>MVPISPIETVPVKLKPGMDGPKVKQWPLTEEKIKALVEICTEMEKEGKISKIGPENPYNTPVFAIKKKDSTKWRKLVDFRELNKRTQDFWEVQLGIPHPAGLKQKKSVTVLDVGDAFYSVPLDKDFRKYTAFTIPSINNETPGIRYQYNVLPMGWKGSPAIFQSSMTKILEPFRKQNPDIVIYQYVDDLYVGSDLEIGQHRTKIEELRQHLLRWGFTTPDKKHQKEPPFLWMGYELHPDKWTVQPIVLPEKDSWTVNDIQKLVGKLNWASQIYAGIKVRQLSKLLRGTKALTEVVPLTEEAELELAENREILKEPVHGVYYDPSKDLIAEIQKQGQGQWTYQIYQEPFKNLKTGKYARMKGAHTNDVKQLTEAVQKIATESIVIWGKTPKFKLPIQKETWEAWWTEYWQATWIPEWEFVNTPPLVKLWYQLEKEPIIGAETFYVDGAANRETKLGKAGYVTDRGRQKVVPLTDTTNQKTELQAIHLALQDSGLEVNIVTDSQYALGIIQAQPDKSESELVSQIIEQLIKKEKVYLAWVPAHKGIGGNEQVDKLVSAG[2x];>[2x]MAHHHHHHALEVLFQGPISPIETVPVK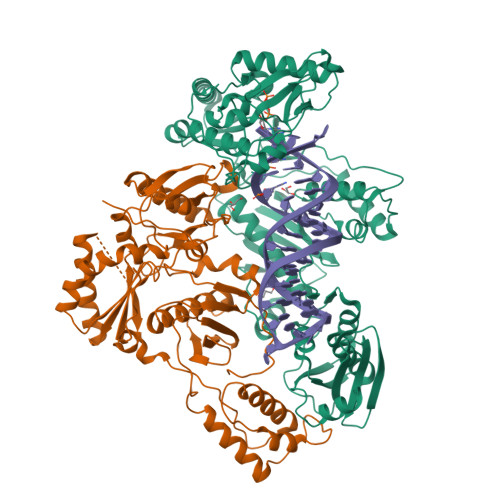LKPGMDGPKVKQWPLTEEKIKALVEICTEMEKEGKISKIGPENPYNTPVFAIKKKDSTKWRKLVDFRELNKRTQDFWEVQLGIPHPAGLKQKKSVTVLDVGDAYFSVPLDKDFRKYTAFTIPSINNETPGIRYQYNVLPQGWKGSPAIFQSSMTKILEPFRKQNPDIVIYQYMDDLYVGSDLEIGQHRTKIEELRQHLLRWGFTTPDKKHQKEPPFLWMGYELHPDKWTVQPIVLPEKDSWTVNDIQKLVGKLNWASQIYAGIKVRQLSKLLRGTKALTEVVPLTEEAELELAENREILKEPVHGVYYDPSKDLIAEIQKQGQGQWTYQIYQEPFKNLKTGKYARMKGAHTNDVKQLTEAVQKIATESIVIWGKTPKFKLPIQKETWEAWWTEYWQATWIPEWEFVNTPPLVKLWYQ> HKKL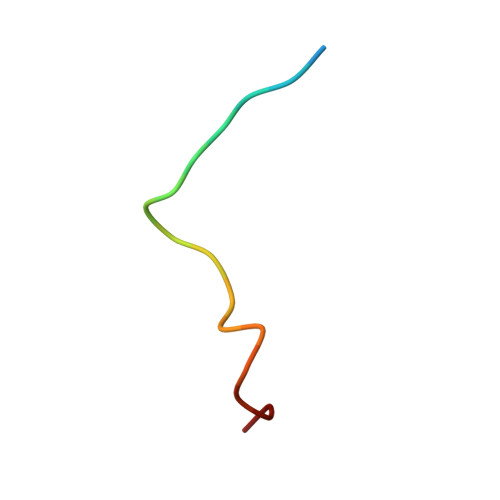VINKDMRTDLFSPPN SpoIIE from B. subtilis is an 827-residue protein thought to consist of three domains. It has 10 putative membrane-spanning segments at its N-terminus and a PP2C-type phosphatase domain at its C-terminus. SpoIIE belongs to the metal-dependent protein phosphatase (PPM) family exemplified by human PP2C. The pathway of σF activation begins with the dephosphorylation of SpoIIAA∼ P by SpoIIE and culminates in the displacement of σF from the complex with SpoIIAB by SpoIIAA.

The crystals appeared from Tris-buffered sodium citrate solutions at pH 8.5 and belong to the space group P6122 with a = b = 89 Å and c = 319 Å. Native data and selenomethionine (SeMet) derivative data at three wavelengths were obtained from these crystals, and the structure was solved by multiwavelength anomalous dispersion (MAD) phasing techniques. The coordinates were refined against data extending to 2.6 Å spacing. There are two molecules (A and B) of SpoIIE(590–827) in the asymmetric unit of the crystal, giving a solvent content of 63%. In the course of building into the electron density maps, it became apparent that SpoIIE(590–827) in the crystal is a domain-swapped dimer with β-strands 1–3 exchanged between subunits. At the dimer interface, a pronounced cavity is formed between the edges of the five-stranded β-sheets. There is a pseudo-2-fold axis of symmetry running through the cavity whose sides are formed by the β1 strands on each of the two subunits of the domain-swapped dimer. This cavity contained a strong feature in the electron density maps that could not be accounted for by protein atoms. A xylose in two half-occupancy alternative conformations could be satisfactorily fitted into this density and refined. We observed a single manganese ion at low occupancy in SpoIIE(590–827) even though the crystals were grown in the presence of MnCl2 (up to 50 mM). One explanation for this is that there will be competition for metal chelation between the protein and citrate (a tricarboxylate), which is present in the crystallization solutions at 0.2 M. Another is that SpoIIE(590–827) binds manganese weakly.

>[2x]GPAMSYRVSTGAAHAAKGGGLVSGDSYSMMELGARKYAAAISDGMGNGARAHFESNETIKLLEKILESGIDEKIAIKTINSILSLRTTDEIYSTLDLSIIDLQDASCKFLKVGSTPSFIKRGDQVMKVQASNLPIGIINEFDVEVVSEQLKAGDLLIMMSDGIFEGPKHVENHDLWMKRKMKGLKTNDPQEIADLLMEEVIRTRSGQIEDDMTVVVVRIDHNTPKWASIPVPAIFQNKQEIS> SMTCPFYKKIPGTGFTVDAFQYGVVEGCTAYFLTHFHSDHYAGLSKHFTFPVYCSEITGNLLKNKLHVQEQYIHPLPLDTECIVNGVKVVLLDANHCPGAVMILFYLPNGTVILHTGDFRADPSMERSLLADQKVHMLYLDTTYCSPEYTFPSQQEVIRFAINTAFEAVTLNPHALVVCGTYSIGKEKVFLAIADVLGSKVGMSQEKYKTLQCLNIPEINSLITTDMCSSLVHLLPMMQINFKGLQSHLKKCGGKYNQILAFRPTGWTHSNKFTRIADVIPQTKGNISIYGIPYSEHSSYLEMKRFVQWLKPQKIIPTVNVGTWKSRSTMEKYFREWKLEAGY

The two human DNA exonucleases containing an MBL-fold are SNM1A (also called DCLRE1A), a factor important for DNA interstrand cross-link (ICL) repair, and SNM1B (also called Apollo or DCLRE1B), a DNA repair factor that also plays an key role in maintaining overhangs at telomeres. The SNM1A and SNM1B/Apollo proteins are both classic 5′-3′ exonucleases, requiring a free 5′-phosphate to initiate digestion, but are members of a class of DNA processing factor family that have not previously been structurally characterized. The protein exhibits two structural domains: the metallo-β-lactamase (MBL) domain, arranged as a sandwich of two mixed β sheets (α/β-β/α); and the β-CASP domain, which is characteristic for a subset of MBL nucleases: CPSF-73, Artemis, SNM1A, Pso2, as well as RNaseJ. An extended active site in both enzymes includes, in addition to the canonical di-zinc catalytic centre, a binding pocket that defines the selectivity for terminal 5′ phosphate, and a wide binding groove which is essential for processivity and for the ability to digest past DNA damage sites.

Structures of SNM1A were solved in two different crystal forms at resolutions of 2.16 and 2.19 Å; the structures are virtually identical, except that crystal form B is lacking two N-terminal amino acids present in form A (RMS difference of 0.57 Å). Structures of SNM1A in two different crystal forms show only a single zinc ion. Comparison with SNM1B shows that all residues involved in zinc coordination are conserved; all are in the correct positions, except for D736 which is a different side-chain rotamer. However, it is likely that the active form of SNM1A also depends on the presence of two zinc ions, as demonstrated by the complete dependence on an aspartate (D736) for nuclease activity that should coordinate the missing zinc. When looking from the direction of the active site, SNM1A is predominantly positive, while SNM1B is only moderately so. Remarkably, the reverse side of both proteins is predominantly negative. The electropositive surface regions in SNM1A, identified with Roman numerals in Figure 1C, can probably be attributed to the following residues and structural features: (I) residues K1022, R1024, K1029, R1032 and the dipole of the last α-helix of SNM1A, which is non-helical in SNM1B; (II) residues R697, K698 and K699; (III) residues K743, H744 and K760; and (IV) K940, K947, K948 in the β-CASP domain. In SNM1B it is well ordered and makes hydrogen bonds (via T257 and S258) to the second tartrate molecule. This segment of the chain is partly disordered in the SNM1A crystal structures; it is possible that the ordered conformation is stabilized by, or dependent upon, the presence of the ligand. A striking difference between SNM1A and SNM1B is that while both are similar in overall structure, they differ markedly in their charge distribution, with SNM1A having a very pronounced area of positive potential surrounding the active site.> MHHHHHHITSLYKKAGSEFALVNKDGHSNWSELIKVKTDLDPYRNVPKDMKTEWKWGQYSSDEPSKAVDGDDSSQFHSQDSAIDKPFIIDMQKAYTIEKLELLFRKNGNGSVKRAEIYSSLDGVTYEKVFSNAEGSDIAPWATDGEVKTINFNKPIKVRYFKIVTKESIGNFLAMREFRPYK

As part of the secreted C. perfringens CAZyme arsenal, the bacterium possesses an open reading frame coding for a 220-kDa family 31 glycoside hydrolase (locus tag CPF_1301 in strain ATCC 13124) with predicted α-glucosidase activity, which will be hereafter referred to as CpGH31. In addition to the N-terminal glycoside hydrolase family 31 catalytic module, CpGH31 comprises two fibronectin-type III modules, three CBM32s, a putative cohesin module, and a bacterial immunoglobulin-like 2 module. Though the putative CBMs, referred to as CBM32-1, CBM32-2, CBM32-3, themselves are not closely related at the amino acid sequence level, a primary structure comparison indicates that they all belong to CBM family 32, an observation that is supported by their overall similar structures as determined by X-ray crystallography. Each CpGH31 CBM32 structure comprised the β-sandwich topology characteristic of this CBM family with a short α-helix and a calcium ion capping one side of each module.

Multi-dimensional heteronuclear NMR experiments were used to map the GalNAc binding site on the apo-CBM32-1 structure, determined to 1.35 Å resolution, as co-crystallization and soaking attempts of CpGH31 CBM32-1 with galacto-configured sugars were unsuccessful. A subset of backbone amide resonances that corresponded to residues primarily grouped to four distinct regions of the CBM32-1 backbone were significantly perturbed upon addition of GalNAc, including Gln971, Tyr972, Ser973, Asp975; His990, Ser991, Gln992, Asp993, Leu1015, Gly1021, Asn1022, Gly1023, Ser1024; Ala1087, Met1088, and Glu1090. When mapped onto the apo-CBM32-1 structure, the four regions formed a contiguous site localized to variable loops located at the apex of the CBM, comprising an aromatic residue (Tyr972) and several polar residues (Gln971, Asp975, Ser973, His990, Gln992, Asp993, and Asn1022), consistent with previously identified CBM32 carbohydrate-bindings sites. Saturation transfer difference (STD) NMR spectroscopic analysis revealed strong STD signals for the apolar α- and β-H3, α- and β-H4, α/β-H6, and acetyl group protons whereas the STD signals of the H1 protons were attenuated. These observations suggest that the C1 edge of GalNAc is solvent-exposed and thus accessible for extension of a glycan chain at this position, while the remainder of the sugar would interact with CBM32-1 via hydrophobic and hydrogen bonding contacts. As the crystal structure of CBM32-1 lacks a sugar ligand, the exact role of each of these aromatic residues in coordinating GalNAc is uncertain. However, the secondary aromatic residue (Tyr1774) and binding site histidine (His1671) of the CBM32-3:GalNAc complex described above are structurally conserved with corresponding residues in the binding site of CBM32-1 (Phe1085 and His990, respectively). The other tyrosine residues implicated in both binding sites (Tyr972 in CBM32-1 and Tyr1674 in CBM32-3) are oriented similarly despite being located on different variable loops.> EKPLRKLAFADLLQATNGFHNDSLIGSGGFGDVYKAILKDGSAVAIKKLIHVSGQGDREFMAEMETIGKIKHRNLVPLLGYCKVGDERLLVYEFMKYGSLEDVLHDPKKAGVKLNWSTRRKIAIGSARGLAFLHH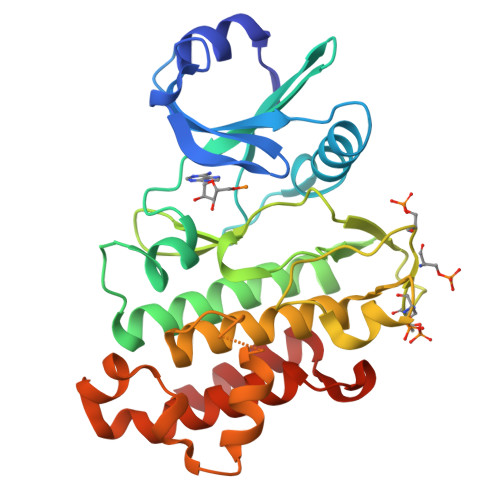NCSPHIIHRDMKSSNVLLDENLEARVSDFGMARLMSAMDTHLSVSTLAGTPGYVPPEYYQSFRCSTKGDVYSYGVVLLELLTGKRPTDSPDFGDNNLVGWVKQHAKLRISDVFDPELMKEDPALEIELLQHLKVAVACLDDRAWRRPTMVQVMAMFKEIQA>[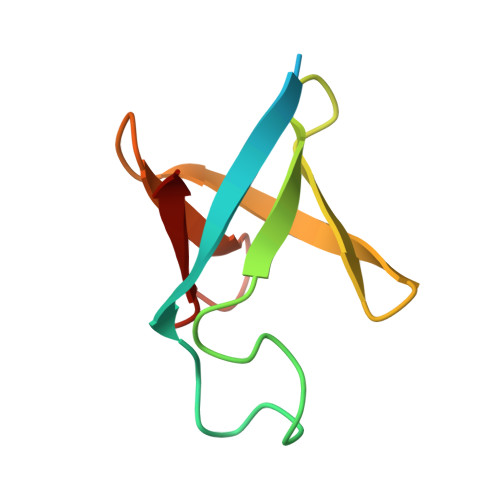6x]MKHHHHHHGSSGMQDQIDAKVIRRNPELTPGIFKKGIEITIDLEEMVCYHSGLTWKVKQLTNTLWSLAGDEHTVMEVI> GAACGACAGTGA;> CGCCGACTC;> TCAGCG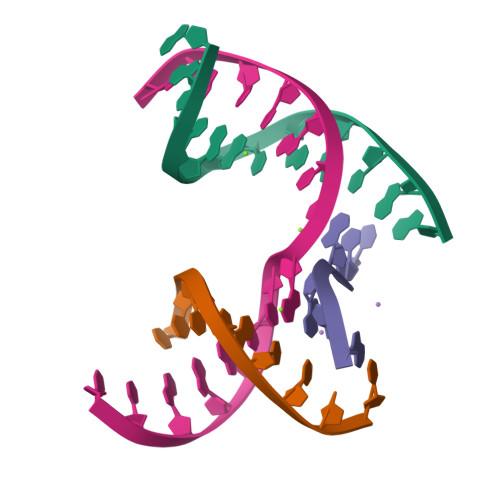;> TCGAGTCGCTGTCGT>CPPKCRCEKLLFYCDSQGFHSVPNALDKGSLGLSLRHNHITELERDQFASFSQLTWLHLDHNQISTVKEDAFQGLYKLKELILSSNKIFYLPNTTFTQLINLQNLDLSFNQLSSLHPELFYGLRKLQTLHLRSNSLRTIPVRLFWDCRSLEFLDLSTNRLRSLARNGFAGLIKLRELHLEHNQLTKINFAHFLRLSSLHTLFLQWNKISNLTCGMEWTWGTLEKLDLTGNEIKAIDLTVFETMPNLKILLMDNNKLNSLDSKILNSLRSLTTVGLSG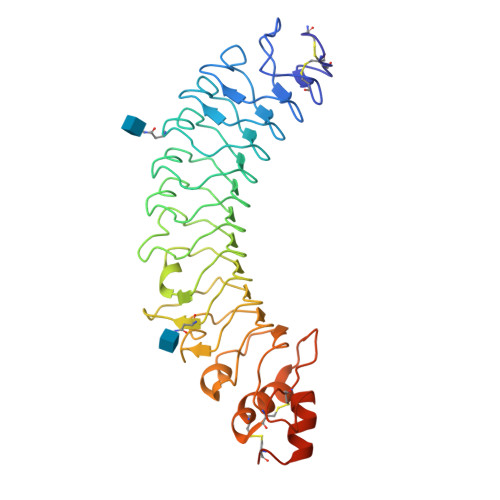NLWECSARICALASWLGSFQGRWEHSILCHSPDHTQGEDILDAVHGFQLCWNLSTTVTVMATTHHHHHH[4x]> GGG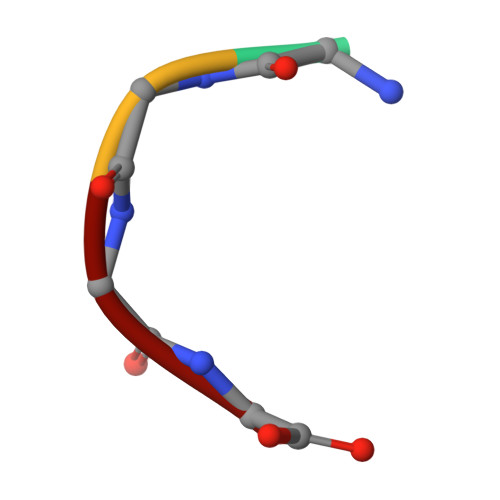G2-fluoro-4-[(2S,3S)-3-hydroxy-2,3-dimethylpyrrolidin-1-yl]-3-methylbenzonitrile 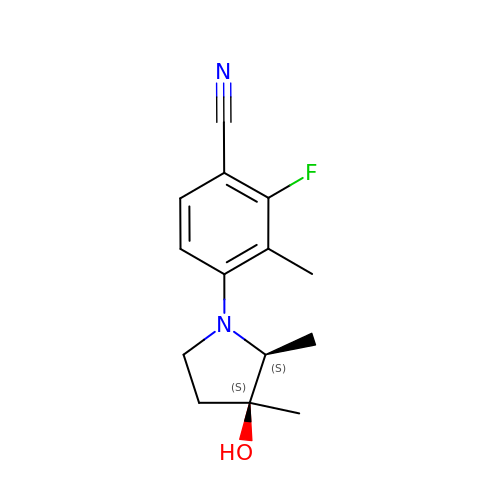| C14 H17 F N2 O | OAXYYUPBCKQHBM-HZMBPMFUSA-N>[6x]GEIAALAVNAWKTTALKNAIAAAQKAGDAAGKIAGESKGVETIIGILEQYYSIYELKGTPLKSFFATTHYTDISNIATVIDTELNTSCGLNSLANQAICGLRTKLGLVAKPGQVMVTQKEAITKMITNVVHKSEITAEAAKTEVAATKTAAAIKMNTEAIEAA;>[6x]HHHHHHQEEDLPRPSISAEPGTVIPLGSHVTFVCRGPVGVQTFR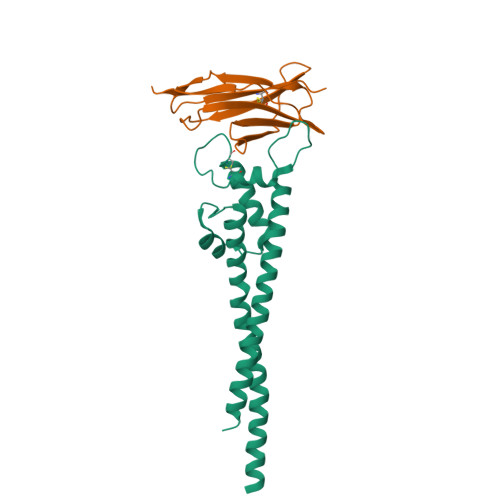LERESRSLYSDTEDVSQTSPSESEARFRIDSVSEGNAGPYRCIYYKPPKWSEQSDYLELLVKEAAA>ADKELKFLVVDDESTMRRIVRNLLKELGFNNVEEAEDGVDALNKLQAGGYGFVISDWRMPNMDGLELLKTIRADGAMSALPVLMVTAHAKKENIIAAAQAGASGYVVKPF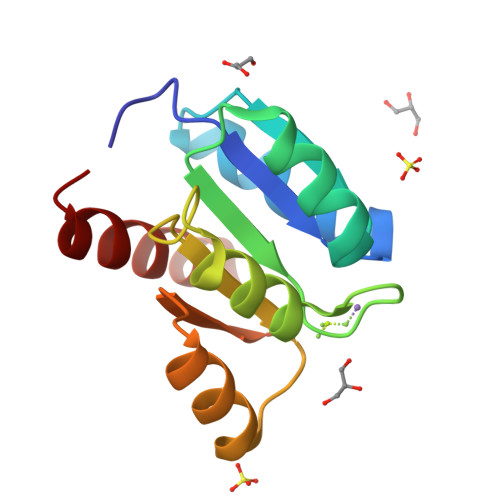TAATLEEKLNKIFEKLGM[2x]> KKLIPILEKIPEVELPVKEITFKEKLKWTGIVLVLYFIMGCIDVYTAGAQIPAIFEFWQTITASRIGTLITLGIGPIVTAGIIMQLLVGSGIIQMDLSIPENRALFQGCQKLLSIIMCFVEAVLFVGAGAFGILTPLLAFLVIIQIAFGSIILIYLDEIVSKYGIGSGIGLFIAAGVSQTIFVGALGPEGYLWKFLNSLIQGVP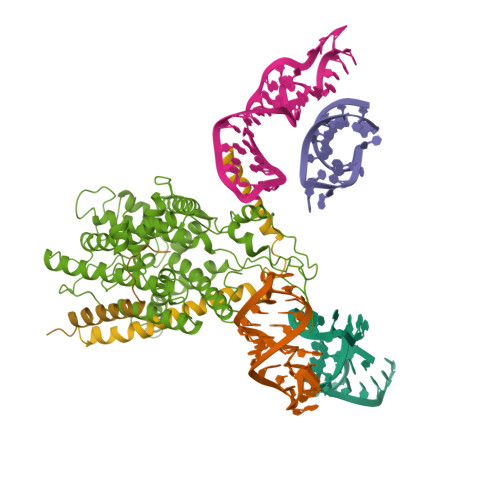NIEYIAPIIGTIIVFLMVVYAECMRRRIVVNYAKRQQGRRVYAAQSTHLPLKVVYVSNIPVILAAALFANIQLWGLALYRMGIPILGHYEGGRAVDGIAYYLSTPYGLSSVISDPIHAIVYMIAMIITCVMFGIFWVETTGLDPKSMAKRIKKSGAFVPGIRPGEQTAKYIEHRLKRYIPPLTVMSSAFVGFLATIANFIGALGGGTGVLLTVSIVYRMYEQLLREKVSELHPAIAKL;> TKGKATVAFAREARTEVRKVIWPTRKPTKDEYLAVAKVTALGISLLGIIGYIIHVPATYIKGILK;> ETFSKIRVKPEHVIGVTVAFVIIEAILTYGRF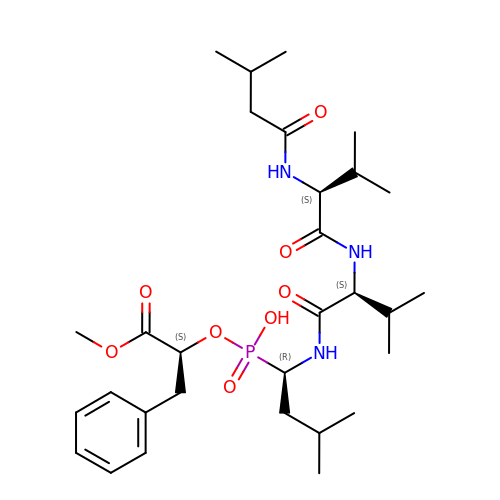N-(3-methylbutanoyl)-L-valyl-N-{(1S)-1-[(R)-[(1R)-1-benzyl-2-methoxy-2-oxoethoxy](hydroxy)phosphoryl]-3-methylbutyl}-L-valinamide | C30 H50 N3 O8 P | ZZHDLOZXEAHENM-KMQNXVAFSA-N>GQYTFSMPSDSHVSSCSEDWVGYQRKCYFISTVKRSWTSAQNACSEHGATLAVIDSEKDMNFLKRYAGREEHWVGLKKEPGHPWKWSNGKEFNNWFNVTGSDKCV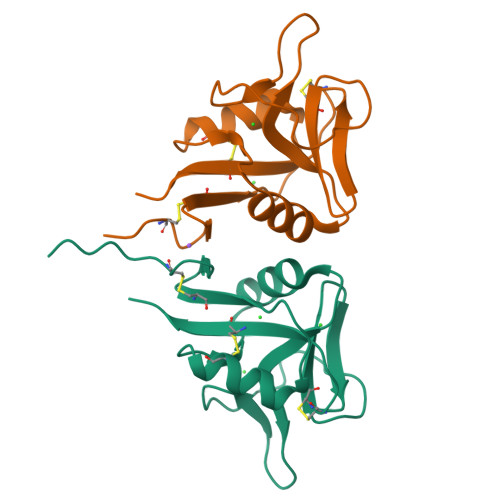FLKNTEVSSMECEKNLYWICNKPYK[2x]>KIFSKCELARKLKSMGMDGFHGYS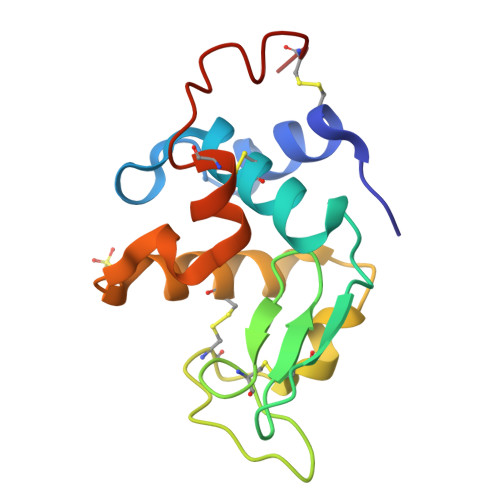LANWVCMAEYESNFNTQAFQGRQSQGSSDYGIFQLNSKWWCKSQSHSSANACNIMCSKFLDDNIDDDIACAKRVVKDPQGMSAWVAWVKHCKGKDLSKYLASCNL[2x]>[4x]IFDKEDYKAFDPELWNAIDAEAERQQNNIELIASENVVSKAVMAAQGTLLTNKTAEGYPGKRYYGGTAVIDVVETLAIERAKKLFGAKFANVQPHSGSQANAAVYMSLIQPGDTVMGMDLSAGGHLTHGAPVSFSGKTYNFVSYNVDKESELLDYDAILAQAKEVRPKLIVAGASAYSRIIDFAKFREIADAV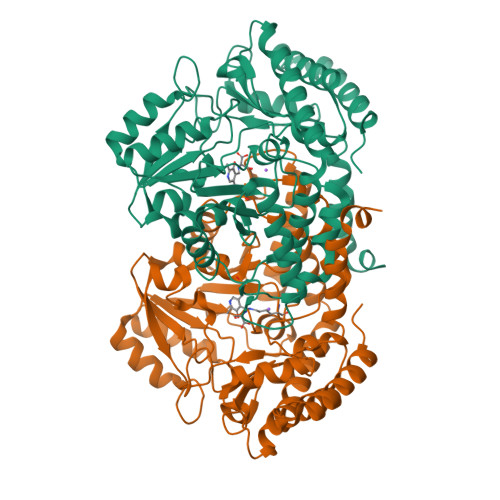GAYLMVDMAHIAGLVASGHHPSPVPYAHVTTTTTHKTLRGPRGGLILTDDEDIAKKLNSAVFPGLQGGPLEHVIAAKAVALKEALDPAFKEYGENVIKNAAAMADVFNQHPDFRVISGGTNNHLFLVDVTKVVENGKVAQNVLEEVNITLNKNSIPYEQLSPFKTSGIRVGSPAITSRGMGEAESRQIAEWMVEALENHDKPEVLERIRGDVKVLTDAFPLY> MENTENSVDSKSIKNLEPKIIHGSESMDS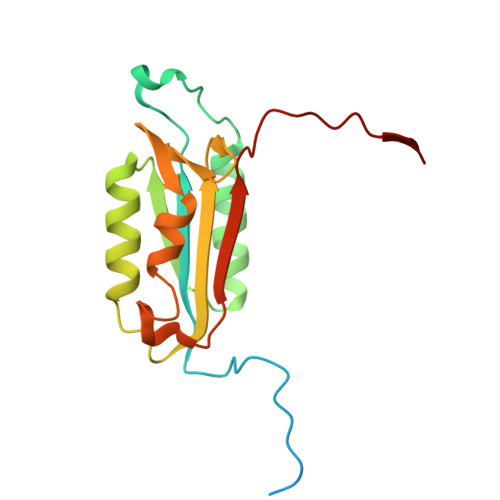GISLDNSYKMDYPEMGLCIIINNKNFHKSTGMTSRSGTDVDAANLRETFRNLKYEVRNKNDLTREEIVELMRDVSKEDHSKRSSFVCVLLSHGEEGIIFGTNGPVDLKKITNFFRGDRCRDLTGKPKLFIIQACRGTELDCGIETD> MKLTDGQIRINHVSSEKKRRELERAIFDELVAVVPDLQPQESRSELIIYLKSLSYLSWLYERNEKLRKQIIAKHE;> DDPVKVRKWKHVQMEKIRRINTKEAFERLIKSVRTPPKENGKRIPKHILLTCVMNDIKSIRSANEALQHILDD

Previous research has demonstrated that Ino2p/Ino4p heterodimer is associated with the transcriptional regulation of phospholipid biosynthetic genes. Mechanistically, Ino2p/Ino4p could specifically recognize the inositol/choline-responsive element (ICRE), followed by the transcription activation of the phospholipid biosynthetic gene. In Saccharomyces cerevisiae, limiting the extracellular level of inositol and choline (IC) leads to the formation of an Ino2p/Ino4p heterodimeric complex, both in vivo and in vitro. The regulation of inositol metabolism is crucial for cellular function. These genes possess at least one copy of the designated inositol/choline-responsive element (ICRE), the consensus sequence (WYTTCAYRTG), or conserved UASINO in their promoter sequence, and they are regulated by their corresponding trans-acting bHLH factors.

Here, we have resolved the crystalline structure of the Ino2pbHLH/Ino4pbHLH/DNA ternary complex at a resolution of 2.25 Å. The crystal belongs to the space group P3121 and contains a single copy of Ino2pDBD/Ino4pDBD-heterodimer-bound promoter DNA (Ino2pDBD/Ino4pDBD/DNA) in the asymmetric unit. The overall structure of the Ino2pDBD/Ino4pDBD/DNA ternary complex reflected that the heterodimer adopts an X-shaped structure while the duplex DNA exhibits the B-type of DNA conformation. Each protein in the heterodimer is comprised of two helices (H1 and H2) separated by a loop, as illustrated in Figure 2. Similarly, the residues in Ino4p include Helix (H1′: Met1′-Val33′), Loop (L’: Val34′-Ser44′), and Helix (H2′: Glu45′-Glu75′). It is note-worthy that the structure reflects the fact that the α-helices (H1 and H1′) of both proteins are symmetrically positioned in the major groove of the promoter DNA. The molecular interaction of protein and DNA might be an important characteristic of transcription factors in regulating various cellular processes, such as gene expression and DNA replication and repair mechanisms. The crystalline structure of the Ino2pDBD/Ino4pDBD/DNA ternary complex indicates that the main interprotein–promoter DNA mutual interactions are mediated by several residues in the first helices (Ino2pH1 and Ino4pH1′), as illustrated in Figure 3A. Our structural analysis highlighted the fact that conserved residues in the basic region of the bHLH domain in Ino2p (Ino2pHis12/Glu16/Arg20/Arg44) and Ino4p (Ino4pHis12/Glu16/Arg19/Arg20) are associated with the sequence-specific recognition of the nucleotides and lies in the major groove of the promoter DNA fragment, which is in agreement with our multiple alignment-sequence results. In order to investigate whether these conserved residues affect the protein–DNA mutual interaction, these residues were mutated to alanine.> ELENIVANTVLLKAREGGGGKRKGKSKKWKEILKFPHISQCEDLRRTIDRDYCSLCDKQPIGRLLFRQFCETRPGLECYIQFLDSVAEYEVTPDEKLGEKGKEIMTKYLTPKSPVFIAQVGQDLVSQTEEKLLQKPCKELFSACAQSVHEYLRGEPFHEYLDSMFFDRFLQWKWLERQPVTKNTFRQYRVLGKGGFGEVCACQVRATGKMYACKRLEKKRIKKRKGESMAL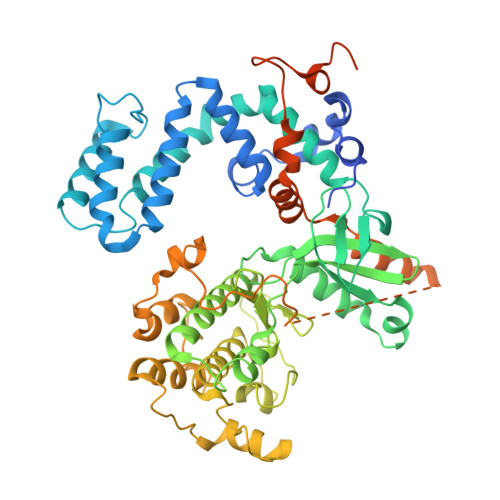NEKQILEKVNSQFVVNLAYAYETKDALCLVLTIMNGGDLKFHIYNMGNPGFEEERALFYAAEILCGLEDLHRENTVYRNLKPENILLDDYGHIRISDLGLAVKIPEGDLIRGRVGTVGYMAPEVLNNQRYGLSPDYWGLGCLIYEMIEGQSPFRGRKEKVKREEVDRRVLETEEVYSHKFSEEAKSICKMLLTKDAKQRLGCQEEGAAEVKRHPFFRNMNFKRLEAGMLDPPFVPDPRAVYCKDVLDIEQFSTVKGVNLDHTDDDFYSKFSTGSVSIPWQNEMIETECFKELNVFGPNGTLPPDLNRNHPPEPPKKGLLQRLFKRQHQNNSKSSPSSKTSFNHHINSNHVSSNSTGSSVDHHHHHH> XMEQLSTANTHFAVDLFRALNESDPTGNIFISPLSISSALAMIFLGTRGNTAAQVSKALYFDTVEDIHSRFQSLNADINKPGAPYILKLANRLYGEKTYNFLADFLASTQKMYGAELASVDFQQAPEDARKEINEWVKGQTEGKIPELLVKGMVDNMTKLVLVNAIYFKGNWQQKFMKEATRDAPFRLNKKDTKTVKMMYQKKKFPYNYIEDLKCRVLELPYQGKELSMIILLPDDIEDESTGLEKIEKQL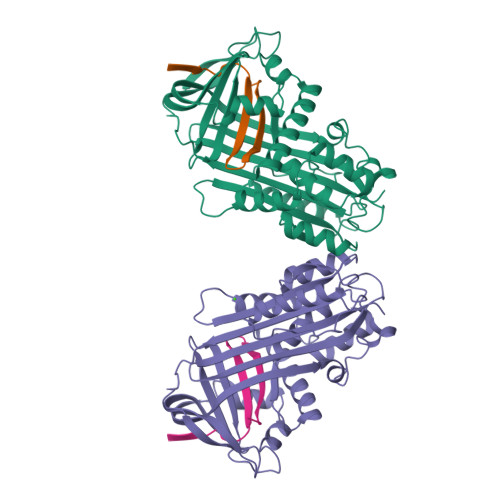TLDKLREWTKPENLYLAEVNVHLPRFKLEESYDLTSHLARLGVQDLFNRGKADLSGMSGARDLFVSKIIHKSFVDLNEEGTEAAAATAGTILLA;> EENFNADHPFIFFIRHNPSANILFLGRFSSP> GSKGRLVIYCSATNVMCENAAKTFEQKYDVKTSFIRNGSGSTFAKIEAEKNNPQADVWYGGTLDPQSQAGELGLLEAYRSPNIDQIMPKFQDPAKVKGNLSSAVYIGILGFAVNTERLKKLGIEKIPQCWNDLTDPKLKGEIQIADPQSSGTAYTAIATFAQLWGEDKAFDYFKHLHPNISQYTKSGITPARNAARGETTVGIGFLHDYALEKEQGAPLEMVVPCEGTGYELGGVSILKGARNLDNAKLFVDFALSKEGQETAWKKGQALQTLTNTTAEQSPLAFDLTKLKLIDYDFEKYGASDERKRLINKWVDEIKLAK

In this study, we investigate AfuABC (Actinobacillus ferric uptake ABC), a BPDT originally identified as an iron-specific transporter in Actinobacillus pleuropneumoniae, a Gram-negative upper respiratory tract pathogen. The locus afuABC encodes 3 polypeptides corresponding to a conventional BPDT–AfuA (a periplasmic binding protein or PBP), AfuB (an inner membrane permease), and AfuC (a cytosolic ATPase). AfuA is a class II/cluster D periplasmic binding protein with two globular α/β domains linked by a dual β-stranded hinge. Instead, AfuABC is a trio of proteins that bind and transport sugar-phosphates such as glucose-6-phosphate (G6P).

To gain insight into the mechanism of ligand capture by this PBP, a structure of apo (open)-AfuA was solved to 1.6Å. The globular domains of apo-AfuA are held at a 29.7° angle relative to the closed form. The binding pocket of AfuA contains both electropositive and electronegative regions, corresponding to the regions of the pocket that bound the phosphate or sugar moiety of G6P respectively. We propose a two-step mechanism for ligand capture by AfuA. Substrates such as G6P or F6P first dock to the protein via hydrogen bonding to residues in the electronegative region of the binding cleft. Next, the negatively charged phosphate group of the ligand serves as the target of a simultaneous rotation and closure of the two globular domains of AfuA, generating a stable AfuA-ligand complex. This cinching mechanism is driven by the electrostatic attraction of the Arg/Lys-rich regions of the binding pocket (which also includes residues such as Ser37 and Thr150).>[4x]MPGEEVSQAKQQLKLIIDPYLSVSEVEKVLAACDFGDLAHTGITRKSGEPYILHPIAVSCILANMRLDPETLMAALLHDVIEDTQYTKDDIIERFGQTVAELVDGVTKLSQSSDKEYNKAASFRKILQATLQDPRVIIIKLADRYHNMTTLGALRPDKRARIAQETFDIFVPMARLVGMNEMADNLENLCYQNLDLDMFDNVQNALLQTKPERCKYQSIWEQNLAELLHNYHIQGRIKKKNNNIELLRHFVKNEMDLQELTHSHAFEIVLQSIA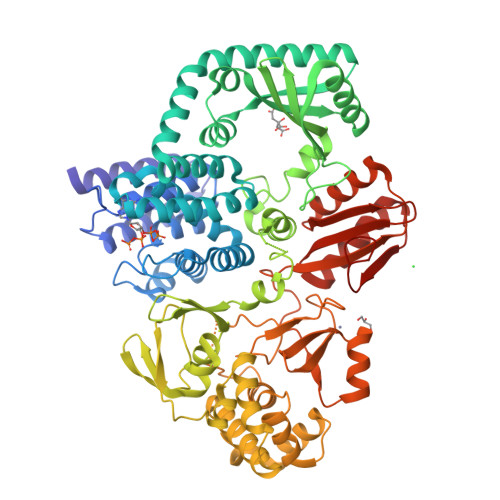DCDRLVAALKENFQVIQYQDHIRRPLPGGNQSLMIKLKGEKTTLSLTIQTELMRKAARFGVVLGENAPQTCRSAIQASMQNLNTLIDGECAKTTFNDLLDYLHQEKIWVYTPHGQLHELPQGATVVDFAYSASLFLGNHAVGAKVDGEIKPLSTPLVSGQVIEIITDVLATPNPDWLSFINTQKARRALQHVLKDQDIEEQRLVGAQALSRALKLFNRSINDLSDADWLDLLQWRHIDNKDALFEQIAVGDLLPQLVANHLFANDKHPRAENSDRLIQGTEGIDVKYAHCCNPILGDPIQGHLTRRGLIVHRIRCHNLLHEQHLHPENIMPLQWKADDVDDVRFTAYLAIYMAMNDEQVSDLIYQCRKNNAGVEMVHSNEQRTFVNIVVNNRKHIAKVIRDLRMHYGFPRIERLDAPAPQMEISKVS>GSMHWNDLLNSNRRKPKNEKKESSQDTSKGRQQIERDYDRILFAAPTRRLADKTQVFPLDKNDSVRTRLTHSHEVANLSRGIGMRLAFELEDDVFKDVSEDICLKRDVPALLAAIGLVHDMGNPPFGHQGEKAMSEWFTKNLPEHSDNYKDKIYGDFRHFDGNSQTLRLVTKLQILNDGYGLNLTYATLASMIKYPRSSESDSSLWKKHGFFLSEKDVVQDIWNNTGLSEGVRHPFTYIMEACDDIAYSVLDAEDIIKKGFASFHDLIDFIQSNQFCKEDDVAKRVIENCKKIHADYAQQKLSPAELNDMSMQMFRVYAIAELVDAVVIAFKDNINEFLNDTCEIKDLISCSSGKNLCQALKKFDSSRGYQHRSVLKLELEGSNYIKGLMDMLWLGIKGRATGDTQYDTPFGRYVYGRISENYRRIFEQENNLPACYKEAQLLADAISGMTDSYLIALHDELRALHQYECRQR[8x]

pmcDeoxynucleoside triphosphohydrolase (dNTPase) enzymes are effector proteins in animal and bacterial cells that hydrolyze dNTP nucleotides and inhibit viral replication. We therefore named the dNTPase-NTase anti-phage defense system Clover and designated the dNTPase protein as Clover protein A (CloA) and the accessory NTase protein as Clover protein B (CloB). Likewise, CloA exhibits strict dGTP substrate specificity, with the activated enzyme only hydrolyzing dGTP and leaving other dNTPs including dTTP unaffected. Together these results demonstrate that CloA is a dGTPase effector that senses phage infection by specifically responding to elevated dTTP concentrations associated with viral replication. Clover defense encodes an accessory enzyme CloB that synthesizes an additional nucleotide signal p3diT that suppresses CloA activation and protects uninfected cells from aberrant nucleotide depletion. p3diT binds to CloA in an allosteric site adjacent to the dTTP binding pocket and raises the threshold of intracellular dNTP levels required to trigger full Clover immune activation.

To define the mechanism of dNTPase-NTase regulation, we determined a 2.4 Å cryo-EM structure of the Salmonella enterica dNTPase protein. The Salmonella dNTPase comprises an N-terminal HD domain and a C-terminal α-helical bundle and forms an octameric complex consisting of four pairs of dimers that arrange to create an architecture resembling a four-leaf clover. The clover-like CloA octameric assembly is formed through extensive interactions across three distinct interfaces. First, HD domain helices α2–α5 interact between adjacent CloA protomers to create anti-parallel dimeric units with α2A, α4A, and α5A forming primarily hydrophobic interactions with α4B, and the α3A residue R46 forming hydrogen-bonding interactions with the peptide backbone of the α3B–α4B loop. Second, CloAAB dimer units multimerize through interactions between the CloAA C-terminal α-helical bundle helices α18C and α22C and helices α6A and α17A that interlock the CloAAC dimer. Third, the CloAAB dimer unit interacts with CloAD, forming pi-stacking interactions between α12 residue H263 of CloAA and CloAD thereby stabilizing the CloAABCD tetramer. Similar to canonical dGTPases like the basal E. coli housekeeping enzyme Dgt, the CloA HD active site motif H117 and D118 coordinate a catalytic Mg2+ ion along with residues H69 and D242, and the HE catalytic dyad H126 and E129 are positioned for substrate dGTP hydrolysis. Interestingly, in contrast to SpdGTPase, no activity was observed with CloA enzyme alone, suggesting that Clover dGTPase activity requires recognition of a cue that occurs during phage infection.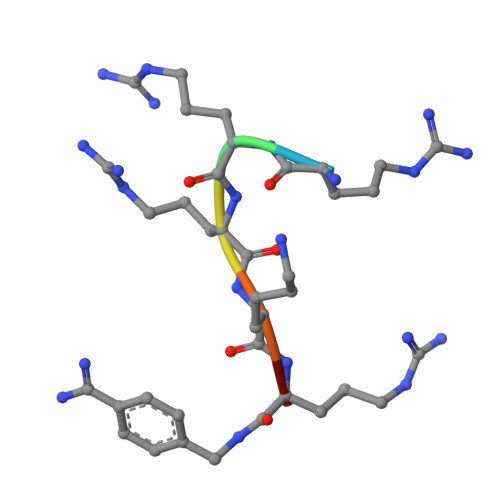> RRRKRX>MIVFVRFNSSHGFPVEVDSDTSIFQLKEVVAKRQGVPADQLRVIFAGKELRNDWTVQNCDLDQQDIVHIVQRPWRKGQEMNATNSFYVYCKGPCQRVQPGKLRVQCSTCRQATLTLTQGPSCWDDVLIPNRMSGECQSPHCPGTSAEFFFKCGAHPTSDKETSVALHLIATNSRNITCITCTDVRSPVLVFQCNSRHVICLDCFHLYCVTRLNDRQFVHDPQLGYSLPCVAGCPNSLIKELHHFRILGEEQYNRYQQYGAEECVLQMGGVLCPRPGCGAGLLPEPDQRKVTCEGGNGLGCGFAFCRECKEAYHEGECSAVFEASGTTTQAYRVDERAAEQARWEAASKETIKKTTKPCPRCHVPVEKNGGCMHMKCPQPQCRLEWCWNCGCEWNRVCMGDHWFDV[2x]

Parkin is an RBR-type ubiquitin ligase which is characterized by RING1, inBetweenRING (IBR) and RING2 domains. Parkin has an N-terminal ubiquitin-like domain (Ubl) that shares 65% sequence similarity with ubiquitin, and a zinc-chelating RING0 domain immediately N-terminal to the RBR domains (Hristova et al, 2009). The RING1 domain recruits E2 enzymes, which carry charged ubiquitin and pass it to a catalytic cysteine in the parkin RING2 domain (Wenzel et al, 2011). Wild-type parkin exists in an autoinhibited state (Chaugule et al, 2011); subsequently, autoinhibition has been demonstrated to be common to RBR ligases (Smit et al, 2012; Stieglitz et al, 2012; Duda et al, 2013).

Phosphorylation of S65 in the Ubl domain enhances parkin activity (Kondapalli et al, 2012). Therefore, we crystallized a version of parkin carrying a negative charge at position 65 (S65DUblR0RBR). This protein, as well as S65EUblR0RBR, showed increased ubiquitination activity compared to wild-type parkin that was further enhanced by phosphoubiquitin in a similar fashion to phosphorylated UblR0RBR. The S65DUblR0RBR crystals grew under the same conditions, with the same unit cell dimensions and crystal packing, as the wild-type UblR0RBR crystals, suggesting little or no structural changes. The structure of S65DUblR0RBR parkin was refined to 2.4 Å, with the same residues present in the density as in the wild-type UblR0RBR crystals. Superposition of S65DUblR0RBR and UblR0RBR (rmsd 0.58 Å) reveals no global conformational changes either in the Ubl domain, or in other parts of the protein (Fig3D). However, close inspection reveals that H227, E300 and H302 of the RING0/RING1 interface are remodelled in the S65DUblR0RBR structure to resemble the interface observed in the truncated R0RBR structures (Fig3E). Interestingly, the remodelling of these residues gives rise to a continuous basic patch comprising K151, H302 and R305 on the surface of Parkin, which is not present when the Ubl domain is unmodified (Fig3F). Since parkin ubiquitination activity is further enhanced through phosphoubiquitin binding, we hypothesized that this basic patch is the phosphoubiquitin-binding site. Taken together, these data suggest that the addition of a negative charge at position 65 of the Ubl domain alters the surface of parkin at the RING0/RING1 interface to facilitate optimal pUb binding.> GSHMRANELQLRWQEYRELVLLLLQWMRHHTAAFEERRFPSSFEEIEILWSQFLKFKEMELPAKEADKNRSKGIYQSLEGAVQAGQLKVPPGYHPLD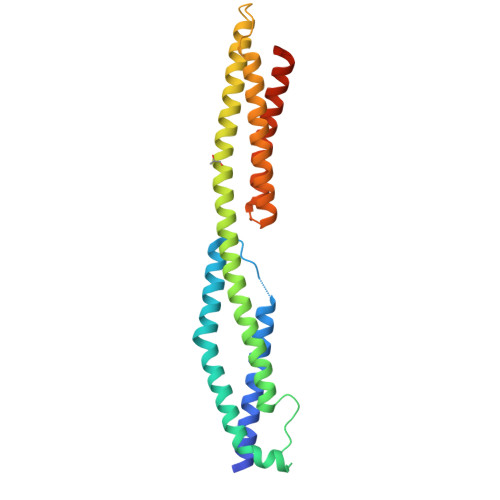VEKEWGKLHVAILEREKQLRSEFERLEALQRIVTKLQMEAGLAEEQLNQADALLQSDVRLLAAGKVPQRAGEVERDLDKADSMIRLLFNDVQTLKDGRHPQGEQMYRRVYRLHKRLVAIRTEYNLRLKAGVAAPATQV> MIFAVRTMVGQEKNIAGLMASRAEKEQLDVYSILASESLKGYVLVEAETKGDVEELIKGMPRVRGIVPGTIAIEEIEPLLTPKKIIENIEKGDVV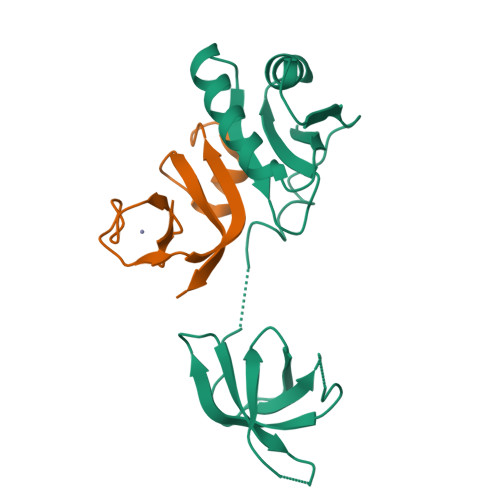EIIAGPFKGERAKVIRVDKHKEEVTLELENAAVPIPITLPVEGVKIVSKHKD;> MGSSHHHHHHSQDPRACLKCKYLTNDEICPICHSPTSENWIGLLIVINPEKSEIAKKAGIDIKGKYALSVKE>MSIAVGMIETLGFPAVVEAADSMVKAARVTLVGYEKIGSGRVTVIVRGDVSEVQASVTAGIENIRRVNGGEVLSNHIIARPHENLEYVLPILE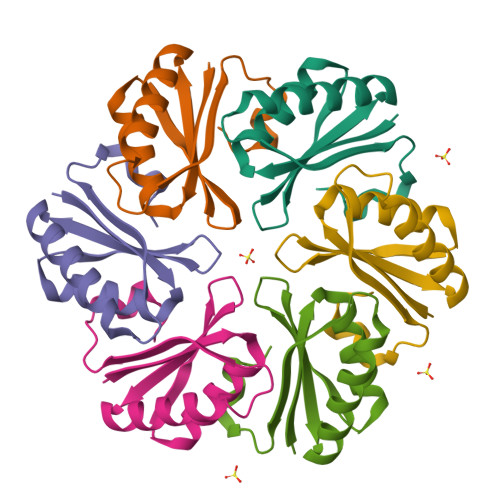HHHHHH[6x]PrimPol is a human DNA polymerase-primase that localizes to mitochondria and nucleus and bypasses the major oxidative lesion 7,8-dihydro-8-oxoguanine (oxoG) via translesion synthesis, in mostly error-free manner. PrimPol is important for both nuclear and mtDNA replication and belongs to the archaeo-eukaryotic primase-polymerase family that differs from other DNA polymerases by possessing a primase activity. The PrimPol catalytic core clasps the template-primer by two α/β modules, ModN and ModC. ModN (residues 35−105) interacts primarily with the template DNA strand and the template oxoG base, whereas ModC (residues 108−200 and 261−348) carries the catalytic residues Asp114, Asp116, and Glu280 and interacts with the incoming dCTP nucleotide: functions normally associated with the finger and palm domains of DNA polymerases, respectively.

To produce the insertion ternary PrimPol complexes with the correct C incoming nucleotide triphosphate opposite the oxoG lesion, we crystallized the catalytic core of human PrimPol (residues 1−354) with a 17-nucleotide (nt) DNA template (5′-CA(oxoG)CGCTACCACACCCC-3′) and a 2′-deoxy-3′-terminated 12 nt DNA primer (5′-GGTGTGGTAGCG-3′) in the presence of dCTP. The overall structure of the PrimPol complex depicting insertion of the correct C opposite the template oxoG residue (oxoG•dCTP) is refined to 2.60 Å resolution and is similar to the structure of the unmodified complex (T-dATP) (root mean square deviation (rmsd) of ~0.35 Å over 249 Cαs of molecule A complexes). Only one ‘metal B’ Ca2+ ion, chelated by the oxygen atoms of the triphosphate tail of dCTP, is observed in the oxoG•dCTP complex despite the intact 3′-OH primer terminus. Somewhat different from the unmodified complex, the N-terminal helix (N-helix; residues 1−17) is slightly shifted (by ~2.5−3 Å) and rotated (by ~3°) away from the major groove of the DNA duplex, allowing for the formation of a salt bridge between the side chains of Arg3 of the N-helix and Glu105, the last C-terminal residue of ModN. The template oxoG base assumes the anti conformation about the glycosidic bond and forms Watson−Crick (WC) interactions with the incoming dCTP. The C1′−C1′ distance in the nascent oxoG(anti)-dCTP base pair is 11 Å, which is slightly longer than the C1′−C1′ distance in the T-dATP pair of the unmodified PrimPol complex (10.4 Å) and in a standard WC pair (10.5 Å). The phosphate group of the oxoG(anti) shifts by ~1.5 Å to avoid a close contact between the O8 and the O5′ atoms of the oxoG residue, and thereby resolving the intrinsic steric clash of the oxoG residue in the anti conformation. Thus, the O8 and the O5′ of the oxoG are now located ~3.5 Å from each other. Since the phosphate group of the template residue in either complex does not make any interactions with PrimPol protein residues, the shift of the phosphate group has little implication for catalytic alignment.

>MNRKWEAKLKQIEERASHYERKPLSSVYRPRLSKPEEPPSIWRLFHRQAQAFNFVKSCKEDVHVFALECKVGDGQRIYLVTTYAEFWFYYKSRKNLLHCYEVIPENAVCKLYFDLEFNKPANPGADGKKMVALLIEYVCKALQELYGVNCSAEDVLNLDSSTDEKFSRHLIFQLHDVAFKDNIHVGNFLRKILQPALDLLGSEDDDSAPETTGHGFPHFSEAPARQGFSFNKMFTEKATEESWTSNSKKLERLGSAEQSSPDLSFLVVKNNMGEKHLFVDLGVYTRNRNFRLYKSSKIGKRVALEVTEDNKFFPIQSKDVSDEYQYFLSSLVSNVRFSDTLRILTCEPSQNKQK[2x]>[2x]HMHHHHHHGGIGQLGLDVWKAAAIKAATEYALTEGAAKGLAAGNAHGMNIVIYHLKELLIDKLVPNICKTVSSTGDYTRVINFSKLIIQKRGAMCGADGGTLSKDMCTQININLGTVLRNGKANLPDKEAVPKVLNRLVSQADKAANEVAKDTSQSVAVKITEQQTAAINATYTS;>[2x]HMHHHHHHQEEDLPRPSISAEPGTVIPLGSHVTFVCRGPVGVQTF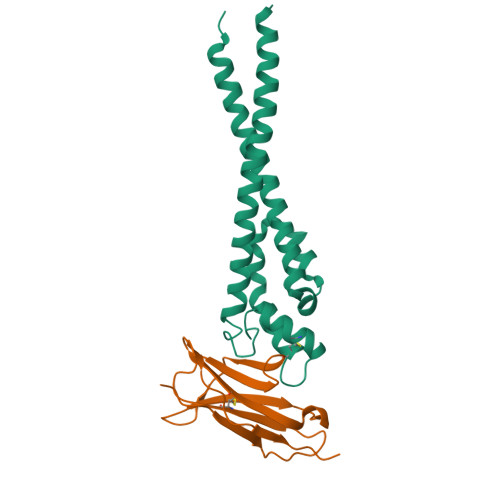RLERESRSTYNDTEDVSQASPSESEARFRIDSVSEGNAGPYRCIYYKPPKWSEQSDYLELLVKEAAA> GPHMLEREKIYQWINEL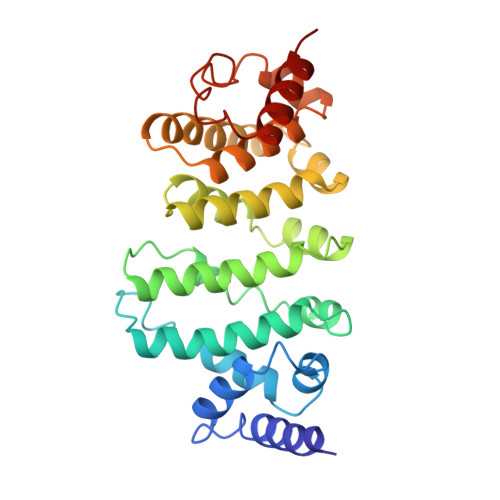SSPETRENALLELSKKRESVPDLAPMLWHSFGTIAALLQEIVNIYPSINPPTLTAHQSNRVCNALALLQCVASHPETRSAFLAAHIPLFLYPFLHTVSKTRPFEYLRLTSLGVIGALVKTDEQEVINFLLTTEIIPLCLRIMESGSELSKTVATFILQKILLDDTGLAYICQTYERFSHVAMILGKMVLQLSKEPSARLLKHVVRCYLRLSDNPRAREALRQCLPDQLKDTTFAQVLKDDTTTKRWLAQLVKNLQE> GPMELAHREYQAGDFEAAERHCMQLWRQEPDNTGVLLLLSSIHFQCRRLDRSAHFSTLAIKQNPLLAEAYSNLGNVYKERGQLQEAIEHYRHALRLKPDFIDGYINLAAALVAAGDMEGAVQAYVSALQYNPDLYCVRSDLGNLLKALGRLEEAKACYLKAIETQPNFAVAWSNLGCVFNAQGEIWLAIHHFEKAVTLDPNFLDAYINLGNVLKEARIFDRAVAAYLRALSFSPNHAVVHGNLACVYYEQGLIDLAIDTYRRAIELQPHFPDAYCNLANALKEKGSVAEAEDCYNTALRLCPTHADSLNNLANIKREQGNIEEAVRLYRKALEVFPEFAAAHSNLASVLQQQGKLQEALMHYKEAIRISPTFA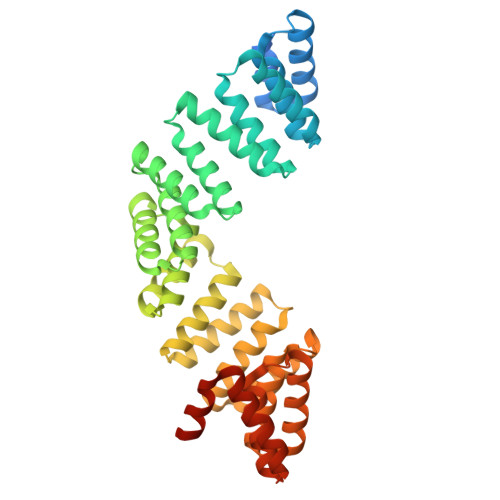DAYSNMGNTLKEMQD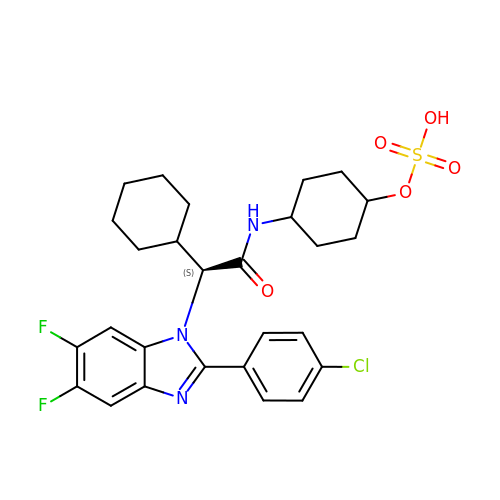trans-4-({(2S)-2-[2-(4-chlorophenyl)-5,6-difluoro-1H-benzimidazol-1-yl]-2-cyclohexylacetyl}amino)cyclohexyl hydrogen sulfate | C27 H30 Cl F2 N3 O5 S | SEHWHKGFYAXJEE-RLSLOFABSA-N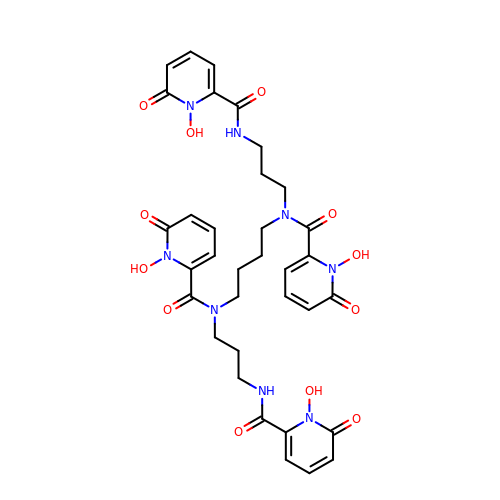N,N'-butane-1,4-diylbis[1-hydroxy-N-(3-{[(1-hydroxy-6-oxo-1,6-dihydropyridin-2-yl)carbonyl]amino}propyl)-6-oxo-1,6-dihydropyridine-2-carboxamide] | C34 H38 N8 O12 | KUWKQASGHNTJAT-UHFFFAOYSA-N> MAQDALSDGFVRLCIDPSLNFFGEGCKILVEGQMTDDGSATPDAVTCVTSELDIIERFGQGSVLTESLRKVFCTCKSGVSVYALPREDAAAGVKAVYTLTIAGPATTDGRVQLYMGEAEYAVDIGVDAGDTATDIAAAIVAAISPDFPYAATAAAGVITLTARNAGTIGNHLSVIYTNLGSCTSVTPEGVTVTFAQTTAGSVNPTPNDYATVVNECCFAVYVLSSDDTDWQENLRDWIR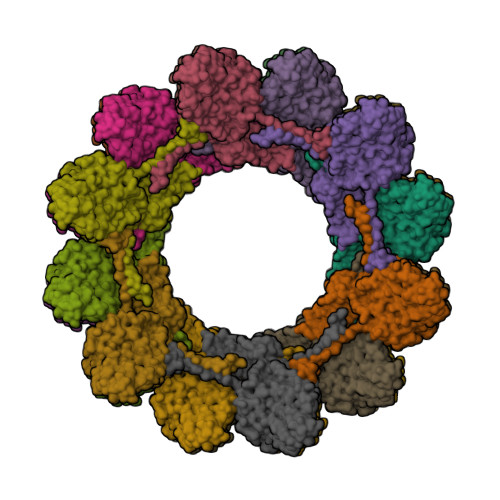SAWDCSKPQCFGHGYVFNKGTLGQVLADGDNSAELSRLALPTTYPVLPYLTNAAYGALSACSTCNNPELNIQGQTFGLLSCINMPESCTPGWTFGEVTQLQANGFVVSGPSTTSGQGNYTSPYIYNDVTNYLRDEKNRPNATFRDASSRRLAAATGVALAEFLQQFNGLAVFTKNTNIRTGIIGTNPRLMLGKIRKWAQDNVGTLFSEFDNINEDIQLLTDFEVQPKCVGQPGIFHLNMRYRPPVRGARINVNMAPALFDNCDR>[2x]MAHHHHHHMTSTATSSPRVITSSPVVVALDYDNRDKALAFVERIDPRDCRLKVGKEMFTLLGPQFVRDLHQRGFEVFLDLKFHDIPNTT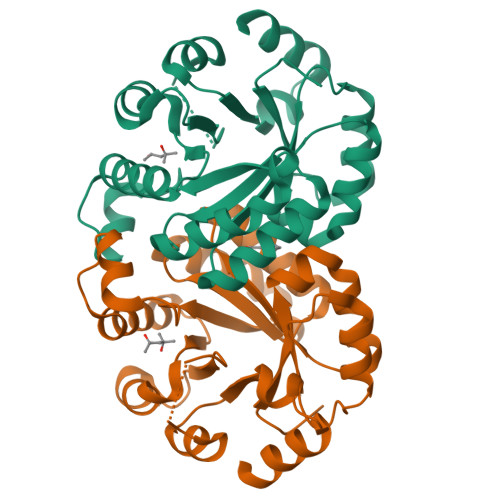ARAVAAAAELGVWMVNVHASGGARMMTAAREALLPFGKEAPLLIAVTVLTSMEASDLQDLGIMLSPADHAAKLAALTKRCGLDGVVCSAQEAVRFKQELGQEFKLVTPGIRPTGSDAGDQRRIMTPEQAQQAGVDYMVIGRPVTQSADPVATLASINASLNKGV> ADFEVHMLNKGKDGAMVFEPASLKVAPGDTVTFIPTDKGHNVETIKGMIPDGAEAFKSKINENYKVTF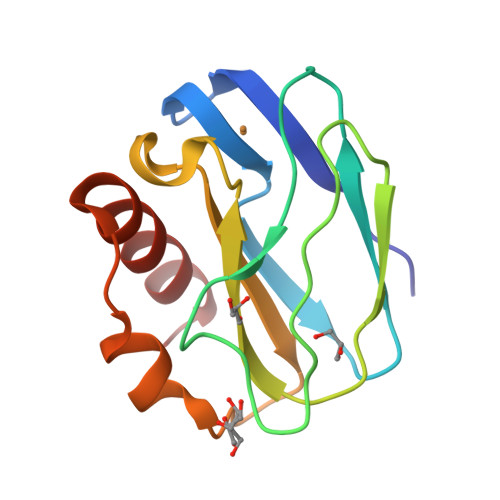TAPGVYGVKCTPHYGMGMVGVVQVGDAPANLEAVKGAKNPKKAQERLDAALAALGN> MGSSHHHHHHGLVPRGSHMDSIQAEEWYFGKI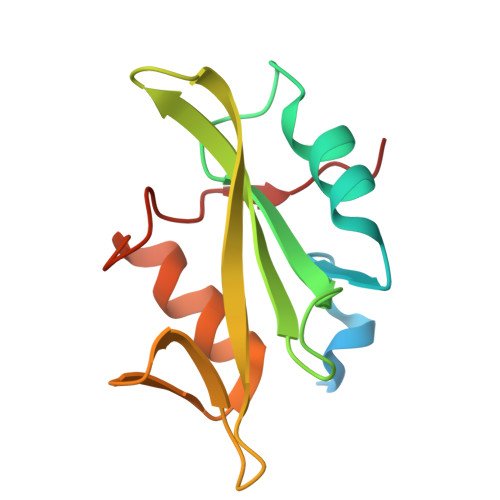TRRESERLLLNAENPRGTFLVRESETVKGAYALSVSDFDNAKGLNVKHYLIRKLDSGGFYITSRTQFNSLQQLVAYYSKHADGLSHRLTTVSPTS>[4x]MSLVAARPLVLVVDDNAVNREALILYLKSRGIDAVGADGAEEARLYLHYQKRIGLMITDLRMQPESGLDLIRTIRASERAALSIIVVSGDTD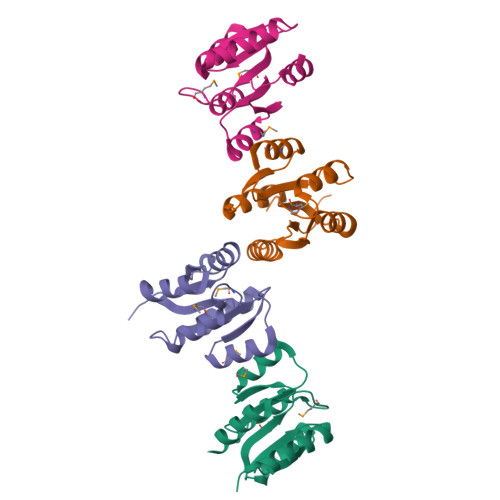VEEAVDVMHLGVVDFLLKPVDLGKLLELVNKELKIGEGHHHHHH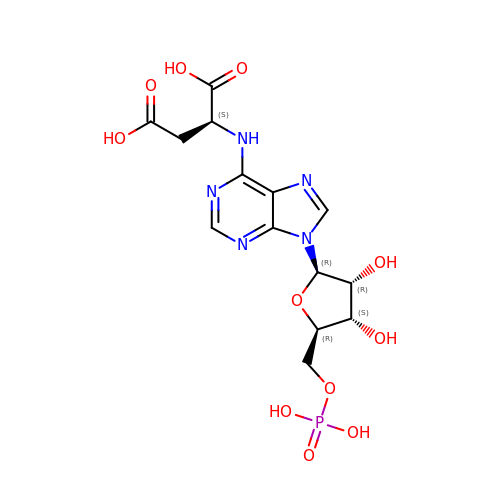2-[9-(3,4-DIHYDROXY-5-PHOSPHONOOXYMETHYL-TETRAHYDRO-FURAN-2-YL)-9H-PURIN-6-YLAMINO]-SUCCINIC ACID | C14 H18 N5 O11 P | OFBHPPMPBOJXRT-VWJPMABRSA-N>[12x]NLQVYP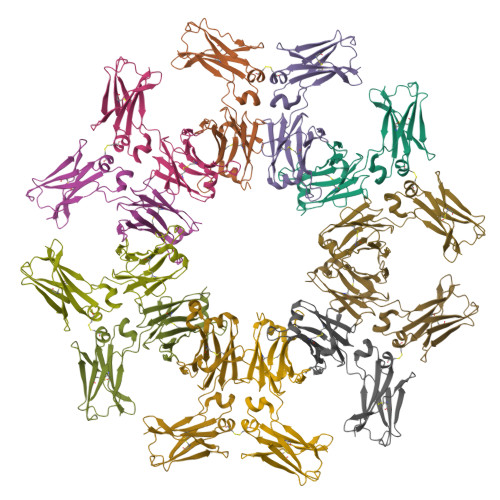LTPTFHDLYFSRNAKITCLVSSMKTIENFDISWEREKAGNLEFVTEDPVLHDNGTYSVASILSVCAEDWESGDKFSCTVRSQDLPSPVKKTIFKQNEGTPKAPDVYLLPPSAQELIQQEMVTLICFVTGFNPKEIFIQWMQGGVSISEDKFINTVPMKSDGEQTYFIYSKLAIPAAKWNQGDVFTCVVGHEALPLYITQQSIDKSSG>[2x]MLEGKVKWFNSEKGFGFIEVEGQDDVFVHFSAIQGEGFKTLEEGQAVSFEIVEG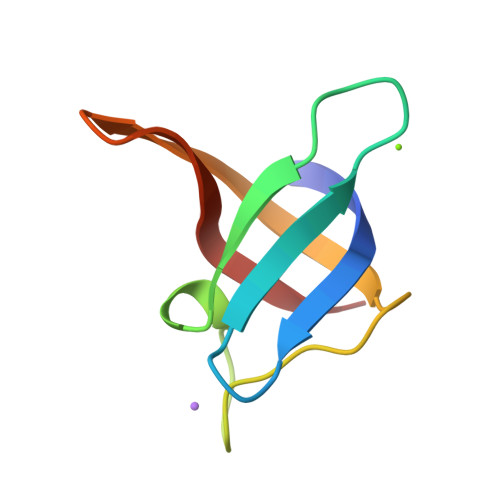NRGPQAANVTKEA> DWNNQSIIKAGERQHGIHIKQSDGAGVRTATGTTIKVSGRQAQGVLLENPAAELRFQNGSVTSSGQLFDEGVRRFLGTVTVKAGKLVADHATLANVSDTRDDDGIALYVAGEQAQASIADSTLQGAGGVRVERGANVTVQRSTIVDGGLHIGTLQPLQPEDLPPSRVVLGDTSVTAVPASGAPAAVSVFGANELTVDGGHITGGRAAGVAAMDGAIVHLQRATIRRGDAPAGGAVPGGAVPGGAVPGGFGPLLDGWYGVDVSDSTVDLAQSIVEAPQLGAAIRAGRGARVTVSGGSLSAPHGNVIETGGGARRFPPPASPLSITLQAGARAQGRALLYRVLPEPVKLTLAGGAQGQGDIVATELPPIPGASSGPLDVALASQARWTGATRAVDSLSIDNATWVMTDNSNVGALRLASDGSVDFQQPAEAGRFKVLMVDTLAGSGLFRMNVFADLGLSDKLVVMRDASGQHRLWVRNSGSEPASANTMLLVQTPRGSAATFTLANKDGKVDIGTYRYRLAANGNGQWSLVGAKA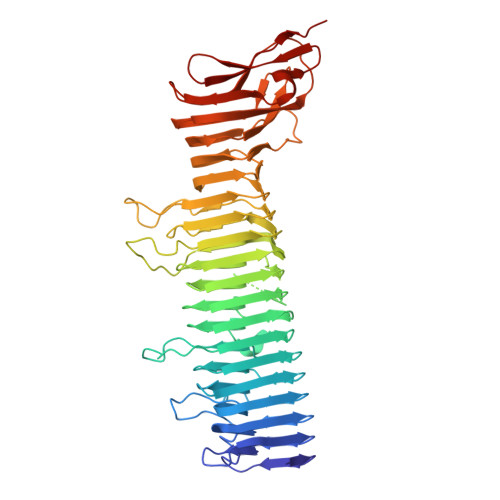PP> MGSSSTQVLVRNATSNDNHQVSKDSLIELAEKSYDSADFFEIMDMLDKRLNDKGKYWRHIAKALTVI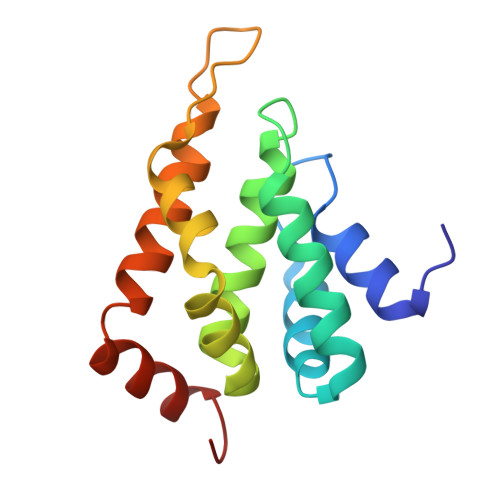DYLIRFGSENCVLWCRENLYIIKTLKEFRHEDDEGIDQGQIVRVKAKELTALLSDDERLNEERNMNIKGR>GKRSERQQADMEMMKDRFAKLLLGEDMSGGGKGVSSALALSNAITNLAASIFGEQTKLQPMPQDRQARWKKEIDWLLSVTDHIVEFVPSQQTSKDGVCTEIMVTRQRGDLLMNIPALRKLDAMLIDTLDNFRGHNEFWYVSRDSEEGQQARNDRTNDKWWLPPVKVPPGGLSEPSRRMLYFQKDSVTQVQKAAMAINAQVLSEMEIPESYIDSLPKNGRASLGDSIYKSITEEWFDPEQFLAMLDMSTEHKVLDLKNRIEASVVIWKRKLHTKDT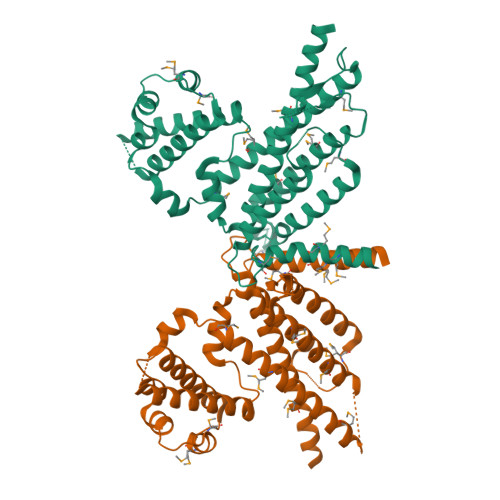KSSWGSAVSLEKRELFEERAETILVLLKQKFPGLPQSSLDISKIQFNKDVGQAVLESYSRILESLAYTVMSRIEDVLYTDTLALKQTLLA[2x]>[2x]GAAAGGGGAGUAGCGUCGG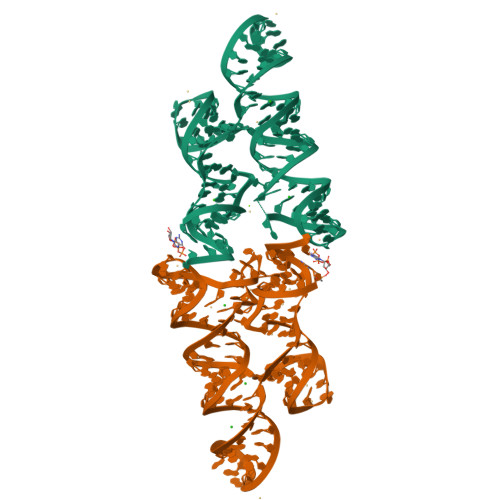GAAACCGAAACAAAGUCGUCAUUACGUGAGGAAACUCACCGGCUUUGUUGACAUACGAAAGUAUGUUUAGCAAGACCUUUCC> NREEKILNREIGFAIGMPVCEFDMVKDPEVQDFRRNILNVCKEAVDLRDLNSPHSRAMYVYPPNVESSPELPKHIYNKLDKGQIIVVIWVIVSPNNDKQKYTLKINHDCVPEQVIAEAIRKKTRSMLLSSEQLKLCVLEYQGKYILKVCGCDEYFLEKYPLSQYKYIRSCIMLGRMPNLMLMAKESLYSQLPMDCFTMPSYSRRISTATPYMNGETSTKSLWVINSALRIKILCATYVNVNIRDIDKIYVRTGIYHGGEPLCDNVNTQRVPCSNPRWNEWLNYDIYIPDLPRAARLCLSICSVKGRKGAKEEHCPLAWGNINLFDYTDTLVSGKMALNLWPVPHGLEDLLNPIGVTGSNPNKETPCLELEFDWFSSVVKFPDMSVIEEHANWSVSREAGFSYSHAGLSNRLARDNELRENDKEQLKAISTRDPLSEITEQEKDFLWSHRHYCVTIPEILPKLLLSVKWNSRDEVAQMYCLVKDWPPIKPEQAMELLDCNYPDPMVRGFAVRCLEKYLTDDKLSQYLIQLVQVLKYEQYLDNLLVRFLLKKALTNQRIGHFFFWHLKSEMHNKTVSQRFGLLLESYCRACGMYLKHLNRQVEAMEKLINLTDILKQEKKDETQKVQMKFLVEQMRRPDFMDALQGFLSPLNPAHQLGNLRLEECRIMSSAKRPLWLNWENPDIMSELLFQNNEIIFKNGDDLRQDMLTLQIIRIMENIWQNQGLDLRMLPYGCLSIGDCVGLIEVVRNSHTIMQIQCKGGLKGALQFNSHTLHQWLKDKNKGEIYDAAIDLFTRSCAGYCVATFILGIGDRHNSNIMVKDDGQLFHIDFGHFLDHKKKKFGYK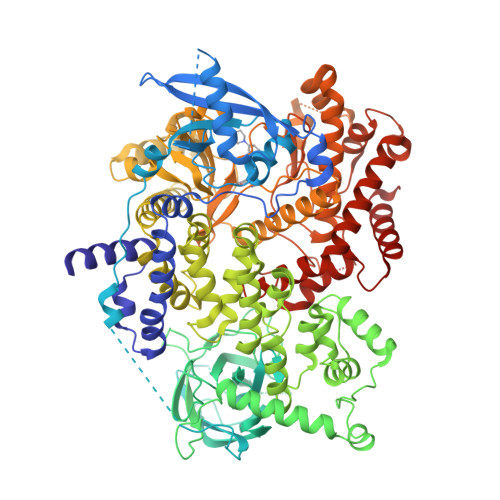RERVPFVLTQDFLIVISKGAQECTKTREFERFQEMCYKAYLAIRQHANLFINLFSMMLGSGMPELQSFDDIAYIRKTLALDKTEQEALEYFMKQMNDAHHGG> MARLEAAVTQSPRNKVAVTGEKVTLSCKQTNSYFNNMYWYRQDTGHELRLIFMSHGI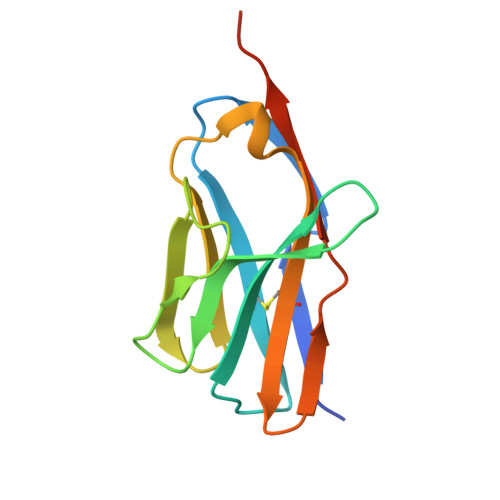RNVEKGDIPDGYKASRPSQENFSLILELATPSQTSVYFCASGGGGTLYFGAGTRLSVLYGSSRVDLQP> MAGLPEARKLLGLAYPERRRLAAAVGFLTMSSVISMSAPFFLGKIIDVIYTNPTVD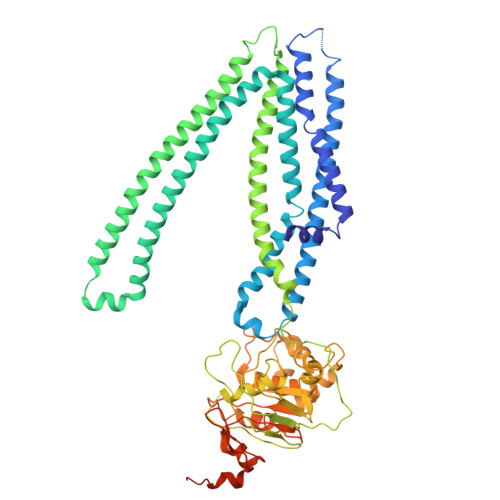YSDNLTRLCLGLSAVFLCGAAANAIRVYLMQTSGQRIVNRLRTSLFSSILRQEVAFFDKTRTGELINRLSSDTALLGRSVTENLSDGLRAGAQASVGISMMFFVSPNLATFVLSVVPPVSIIAVIYGRYLRKLTKVTQDSLAQATQLAEERIGNVRTVRAFGKEMTEIEKYASKVDHVMQLARKEAFARAGFFGATGLSGNLIVLSVLYKGGLLMGSAHMTVGELSSFLMYAFWVGISIGGLSSFYSELMKGLGAGGRLWELLEREPKLPFNEGVILNEKSFQGALEFKNVHFAYPARPEVPIFQDFSLSIPSGSVTALVGPSGSGKSTVLSLLLRLYDPASGTISLDGHDIRQLNPVWLRSKIGTVSQEPILFSCSIAENIAYGADDPSSVTAEEIQRVAEVANAVAFIRNFPQGFNTVVGEKGVLLSGGQKQRIAIARALLKNPKILLLDQATSALDAENEYLVQEALDRLMDGRTVLVIAHRLSTIKNANMVAVLDQGKITEYGKHEELLSKPNGIYRKLMNKQSFISAENLYFQGDYKDDDDKHHHHHHHHHH>MDKKELFDTVINLEEQIGSLYRQLGDLKQHIGEMIEENHHLQLENKHLRKRLDDTTQQIEKF[2x]

The main regulatory protein YabA was also found to prevent over-initiation by inhibiting the cooperative binding of DnaA to oriC. Furthermore, YabA downregulates replication initiation as part of a multimeric complex with DnaA and DnaN that is associated with the replication factory. YabA is a small protein of 119 residues, with an unusual predicted organization composed of a leucine zipper at its N-terminus and a putative zinc-binding domain at its C-terminus. Solution studies demonstrated that YabA is a tetramer in which the monomeric CTDs are separated from the tetrameric NTDs by a flexible linker resulting in an extended conformation.

We attempted to crystallize YabA and obtained two crystal forms (form I and II, see ‘Materials and Methods’ section for details). In both cases, analysis of the unit cell contents and lattice interactions indicated that proteolysis occurred during crystallization. The structure obtained with form I crystals was refined to a final resolution of 2.7 Å with good geometry. The crystal structure of the NTD of YabA revealed an extended α-helix, four of which assemble into a helical bundle. The A'B dimer resembles a pair of tweezers assembled via tight interactions of the C-terminal elements of the two helices whose arrangement can be described as a parallel coiled-coil. Two pairs of these tweezers (AB’ and A'B) embrace each other to form the head-to-head tetramer. The tetramer thus comprises a central four-helix bundle flanked by pairs of helical extensions arranged as coiled coils. The four-helix bundle comprises residues 1–35 of the four chains with chains A and B’ running antiparallel to chains A’ and B. The interior of the bundle is formed by the close packing of the aliphatic side chains of L6, V10, L13, I17, L20, L24, L27, I31 and M34 from all four chains creating a substantial hydrophobic core. The heptadic arrangement of L6, L13, L20 and L27 gives rise to a leucine zipper-type interdigitation of side chains projecting from pairs of adjacent chains (A-A’ and B-B’). The flanking coiled-coil regions are formed by the C-terminal halves of chains A and B’ on one side of the four helical region and chains A’ and B on the other (residues 36–62). These pairs of helices, which are splayed in the four helix bundle region, converge at their C-termini where hydrophobic interactions of the side chains of M34, L41, L48, L52 and I59 with the equivalent residues in the partner chain are augmented by hydrogen bonding interactions of the side chains of N38, N45, T55 and most strikingly by reciprocal salt-bridging interactions between the side chains of E44 and R49.> QKTGTAEMSSILEERILGADTSVDLEETGRVLSIGDGIARVHGLRNVQAE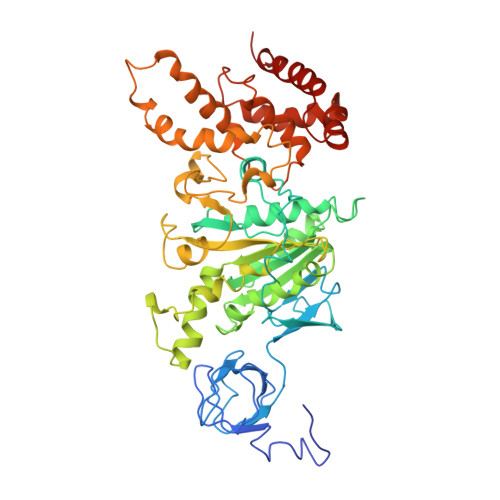EMVEFSSGLKGMSLNLEPDNVGVVVFGNDKLIKEGDIVKRTGAIVDVPVGDELLGRVVDALGNAIDGKGPVGSKIRRRVGLKAPGIIPRISVREPMQTGIKAVDSLVPIGRGQRELIIGDRQTGKTSIAIDTIINQKRFNDGTDEKKKLYCIYVAIGQKRSTVAQLVKRLTDADAMKYTIVVSATASDAAPLQYLAPYSGCSMGEYFRDNGKHALIIYDDLSKQAVAYRQMSLLLRRPPGREAYPGDVFYLHSRLLERAAKMNDSFGGGSLTALPVIETQAGDVSAYIPTNVISITDGQIFLETELFYKGIRPAINVGLSVSRVGSAAQTRAMKQVAGTMKLELAQYREVAAFAQFGSDLDAATQQLLSRGVRLTELLKQGQYSPMAIEEQVAVIYAGVRGYLDKLEPSKITKFESAFLSHVVSQHQSLLGNIRTDGKISEQSDAKLKEIVTNFLAGFEP> GSHMSRKIRDLIESKRFQNVITAIIVLNGAVLGLLTDTTLSASSQNLLERVDQLCLTIFIVEISLKIYAYGVRGFFRSGWNLFDFVIVAIALMPAQGSLSVLRTFRIFRVMRLVSVIPTMRRVVQGMLLALPGVGSVAALLTVVFYIAAVMATNLYGATFPEWFGDLSKSLYTLFQVMTLESWSMGIVRPVMNVHPNAWVFFIPFIMLTTLTVLNLFIGIIVDAMAITKEQEEEAKTGHHQEPISQTLLHLGDRLDRIEKQLAQNNELLQRQQPQKK

Voltage-gated sodium channels (Navs) specifically enable the passage of sodium ions across cell membranes, contributing to the electrical signalling in cells. Mutations in hNavs have been associated with a range of channelopathies, including pain, epilepsy, and heart disorders, making them major targets for drug development. The NavMs channel has been shown to be an excellent exemplar for hNavs as it exhibits highly similar functional, conductance, and drug-binding (similar IC50 values) characteristics, as well as sequence and structural homologies.

CBD is located at the ends of the fenestrations that lie closest to the central pore, and protrudes into (and blocks) the central transmembrane cavity, just below the sodium ion selectivity filter. There is experimental electron density and enough room (third panel from left) for four CBD molecules in this region, although one would be sufficient to block sodium ion passage, as seen from the HOLE depictions and pore radius plots, which show the size of the transmembrane pathway with and without different numbers of CBD molecules; their blockage clearly provides a mechanism for channel inhibition as well as a basis for understanding the concentration-dependence of the drug effects. Each binding site is comprised of 11 residues from three different subunits in NavMs (shown in detail and in different colours in Figure 1D & E). It should be noted here, that this region of the apo structure also exhibits some electron density (but has a different size and shape), which has been attributed to detergent molecules. The (2Fo-Fc) electron density map of the CBD complex clearly indicates that in these crystals the site is occupied by CBD rather than by detergent. The CBD-binding site is a novel site, near to, but not coincident with, known analgesic binding sites in sodium channels. The binding site is located at the pore end of the transmembrane fenestrations which enable the ingress of hydrophobic molecules into the channel lumen, hence this may also provide the pathway for CBD to enter and block the channels.> HHHHHHENLYFQGAADTTYVVAGTTNLTGYEWVGTPDAAPENVMTADGSVFTKTFSAVPAGKNYQLKVVANTGDEQKWIGLDGTDNNVTFDVETACDVTVTFDPATNKITVTGDGVKMVTDLEVNSITVVGNGEDNWLNGVAWGVDAEVNHMTQVSDKVYQIKYENIESADDAYQFKFAANDDWAASWGLPEQSATPIGEEFDL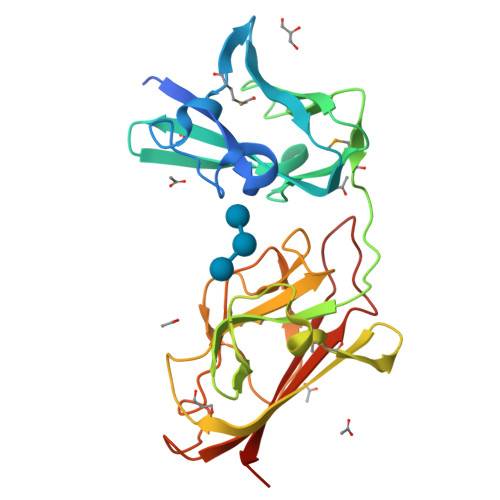TFNGQNMLLNTVSAGFEEDSLVDVTITLDITNFDYSTRSGAKATVKVEPSTP> MSQIIWGAYAQRNTEDHPPAYAPGYKTS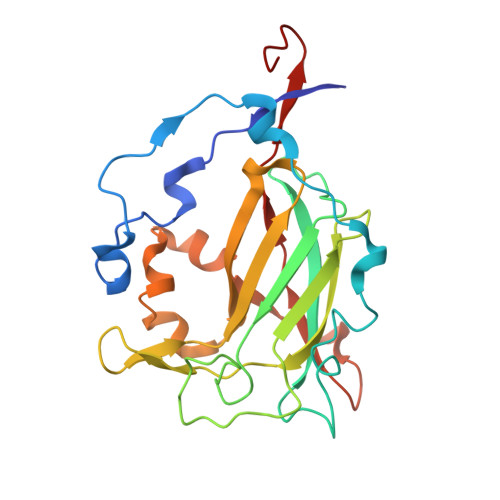VLRSPKNALISIAETLSEVTAPHFSADKFGPKDNDLILNYAKDGLPIGERVIVHGYVRDQFGRPVKNALVEVWQANASGRYRHPNDQYIGAMDPNFGGCGRMLTDDNGYYVFRTIKPGPYPWRNRINEWRPAHIHFSLIADGWAQRLISQFYFEGDTLIDSCPILKTIPSEQQRRALIALEDKSNFIEADSRCYRFDITLRGRRATYFENDLT>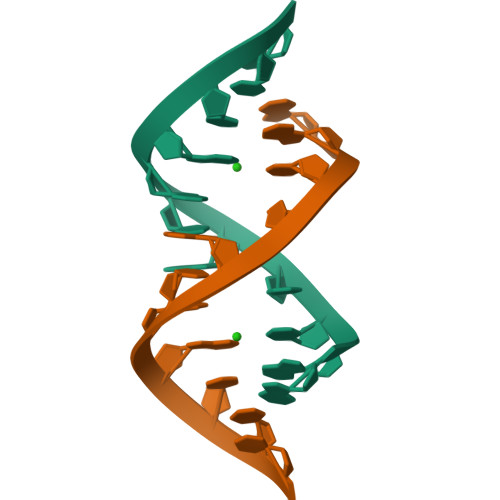[2x]GGUCACAGCCC>SETVVTEVLGHRVTLPCLYSSWSHNSNSMCWGKDQCPYSGCKEALIRTDGMRVTSRKSAKYRLQGTIPRGDVSLTILNPSESDSGVYCCRIEVPGWFNDVK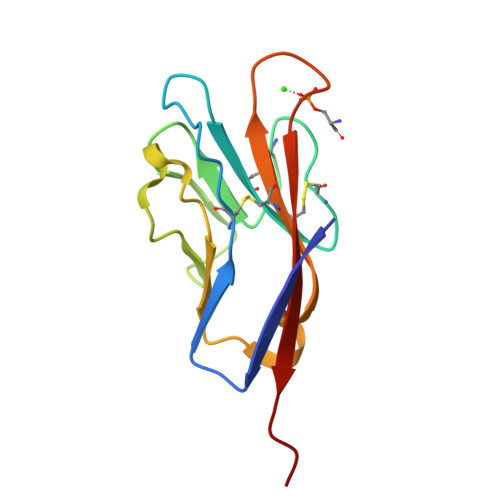INVRLNLQRALV[6x]> NDDKLYRADSRPPDEIKQSGG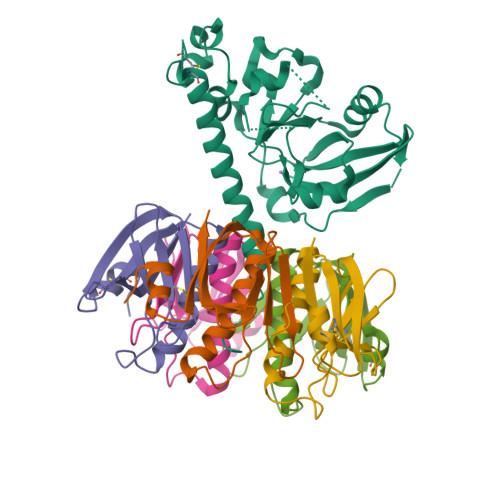LMPRGQSESFDRGTQMNINLYDHARGTQTGFVRHDDGYVSTSISLRSAHLVGQTILSGHSTYYIYVIATAPNMFNVNDVLGAYSPHPDEQEVSALGGIPYSQIYGWYRVHFGVLDEQLHRNRGYRDRYYSNLDIAPAADGYGLAGFPPEHRAWREEPWIHHAPPGCGNAPRSSMSNTCDEKTQSLGVKFLDEYQSKVKRQIFSGYQSDIDTHNRIKDEL;>TPQNITDLCAEYHNTQIHTLNDKIFSYTESLAGKREMAIITFKNGATFQVEVPGSQHIDSQKKAIERMKDTLRIAYLTEAKVEKLCVWNNKTPHAIAAISMAN[5x]> LSYRCPCRFFESHVARANVKHLKILNTPNCALQIV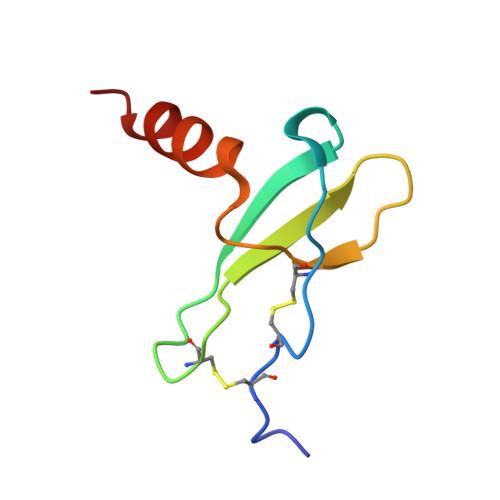ARLKNNNRQVCIDPKLKWIQEYLEKALNK(3R)-1-azabicyclo[2.2.2]oct-3-yl[bis(5-chlorothiophen-2-yl)]methanol 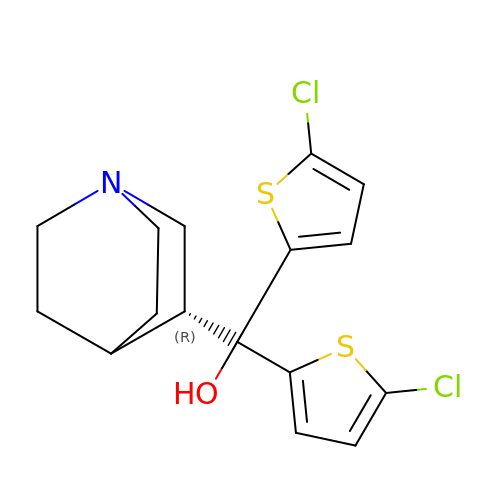| C16 H17 Cl2 N O S2 | ZDHSJVXBNDEQSR-NSHDSACASA-N> MAETKSMFREVLPKQGQLYVEDITTMVLCKPKLLPLKSLTLEKLEKMQQAA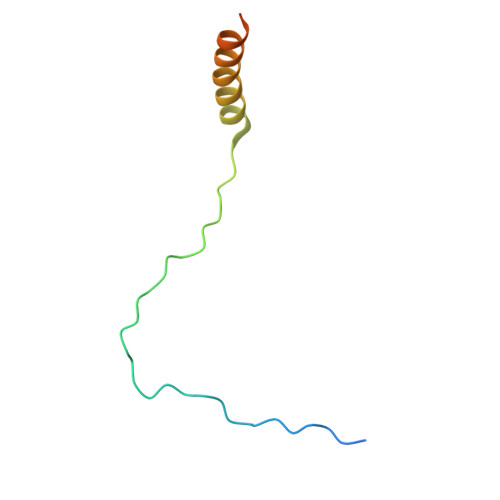QDTIHQQEMTEKEQKITH>HHHHHHSSGLVPRGSHMFRSSLTHLQAASRVFIVGGHITPFVGKGSPLFIDKKHPDFGKKKNMTLEEILATTVQGTMEHSGLSGREGIVDQVVVGNFLGELFSSQGHLGPAAIGSLTYGQAGSKNPLMYKPAMRVEGACASGGLAVISAMNALKSGSADITLAVGVEVQTTASARVGGDYLARAADYQRQRQLDDFTFPCLFAKRMKYIAEHNHFTMEDTARVAAKAYANGNKNPLAHMHTRKLTFEQCNGEDPSNVKFLGNETYKEYLRMTDCSQVSDGGAGVVLANEEGLRKMGLSPNDSRLVEIKSIACAVS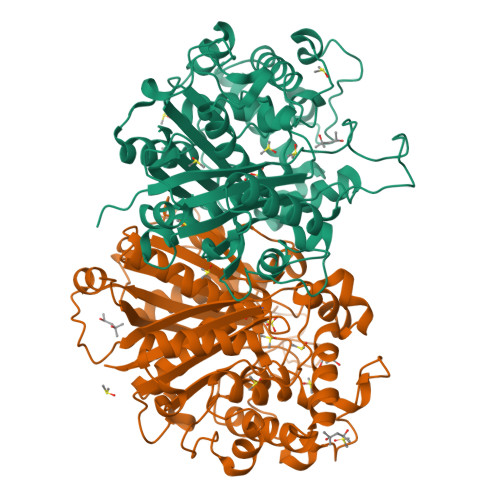NLYEDPDDACCMFTSRQAAQKALSMANIKPSDLNVAEVHDCFTIAEMLMYEALGIAEYGHAKDLIRNGDTTLEGRIPVNTGGGLLSFGHPVGATGIKQIMEVYRQMKGQCEAYQMKKIPALGATLNMGGDDKTAVSAVLQNI[2x]>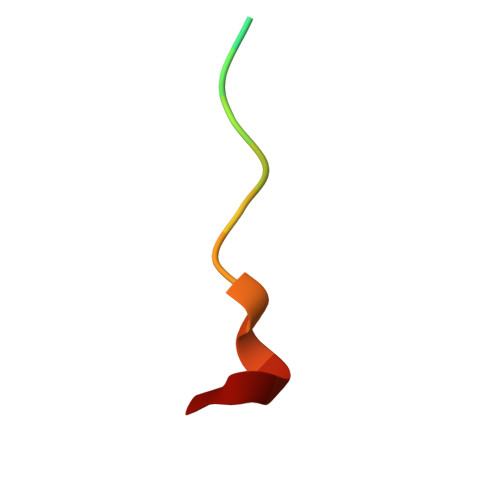 MEHRGPPPEYPFKGM> MPTRKSNTYLSLVNSYLIDSPQPSSINYWWNLGSLLGLCLVIQIASGVFLAMHYSSNIELAFDSVEHIMRDVNAGWLIRYIHANGASFFFICMYLHIGKALYYGSYKQPRVMLWVIGVVIFILTMAIAFMGYCLVYGQMSHWGATVITNLLSAIPFIGNDIVPFIWGGFSVSNPTIQRFFALHFLLPFILAALVCMHLMALHVHGSSNPVGITGNIDRLPMHPYFIFKDLIT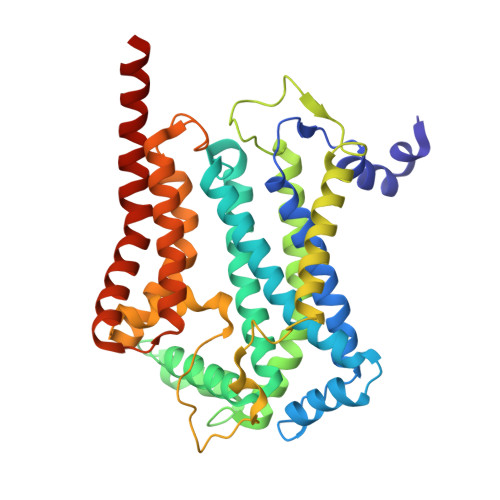VFVFLLIFSLFVFYSPNTLGHPDNYIPGNPMVTPPSIVPEWYLLPFYAILRSIPDKLGGVIAMFGAILILLSLPYTDRSIIRGNSFKVLSKLAFYLFVFNFILLGNLGQLHVEVPYIQLGQFATAYYFAHYIIVVPVISTLENILYYIGTQTRVK(4S)-5-fluoro-4-[({3-hydroxy-2-methyl-5-[(phosphonooxy)methyl]pyridin-4-yl}methyl)amino]pentanoic acid | C13 H20 F N2 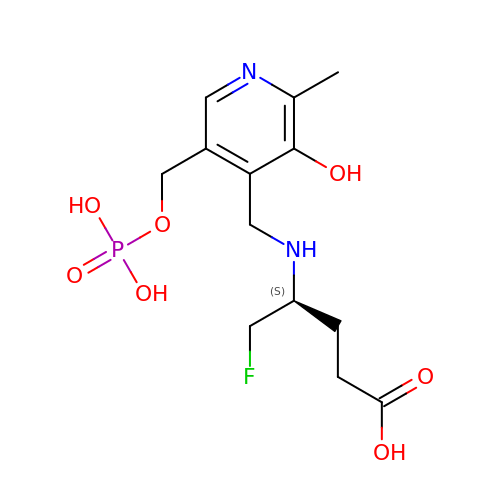O7 P | QWMIOBWBDTXOII-JTQLQIEISA-N> MVDLEQEFALGGRCLAFHGPLMYEAKILKIWDPSSKMYTSIPNDKPGGSSQATKEIKPQKLGEDESIPEEIINGKCFFI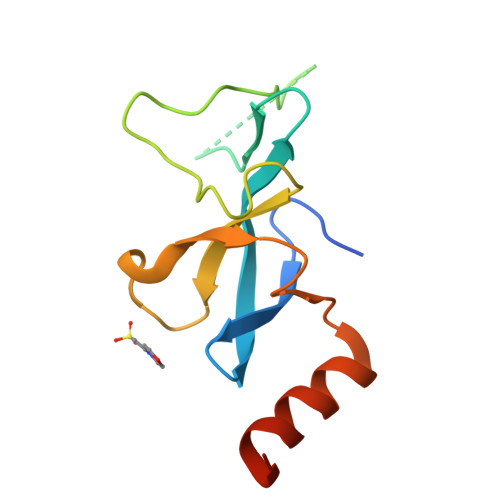HYQGWKSSWDEWVGYDRIRAYNEENIAMKKRLANLEHHHHHH> SAPGEDEECGRVRDFVAKLANNTHQHVFDDLRGSVSLSWVGDSTGVILVLTTFHVPLVIMTFGQSKLYRSEDYGKNFKDITDLINNTFIRTEFGMAIGPENSGKVVLTAEVSGGSRGGRIFRSSDFAKNFVQTDLPFHPLTQMMYSPQNSDYLLALSTENGLWVSKNFGGKWEEIHKAVCLAKWGSDNTIFFTTYANGSCKADLGALELWRTSDLGKSFKTIGVKIYSFGLGGRFLFASVMADKDTTRRIHVSTDQGDTWSMAQLPSVGQEQFYSILAANDDMVFMHVDEPGDTGFGTIFTSDDRGIVYSKSLDRHLYTTTGGETDFTNVTSLRGVYITSVLSEDNSIQTMITFDQGGRWTHLRKPENSECDA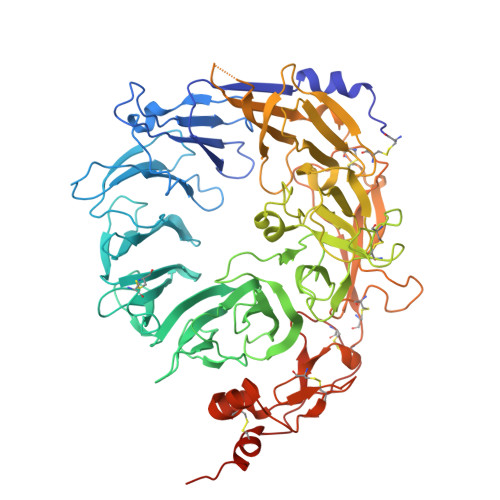TAKNKNECSLHIHASYSISQKLNVPMAPLSEPNAVGIVIAHGSVGDAISVMVPDVYISDDGGYSWTKMLEGPHYYTILDSGGIIVAIEHSSRPINVIKFSTDEGQCWQTYTFTRDPIYFTGLASEPGARSMNISIWGFTESFLTSQWVSYTIDFKDILERNCEEKDYTIWLAHSTDPEDYEDGCILGYKEQFLRLRKSSMCQNGRDYVVTKQPSICLCSLEDFLCDFGYYRPENDSKCVEQPELKGHDLEFCLYGREEHLTTNGYRKIPGDKCQGGVNPVREVKDLKKKCTSNFLSPEKQNSKSNSHHHHHH> MLTEGISIQSYDGHTFGALVGSPAKAPAPVIVIAHEILGVNAFM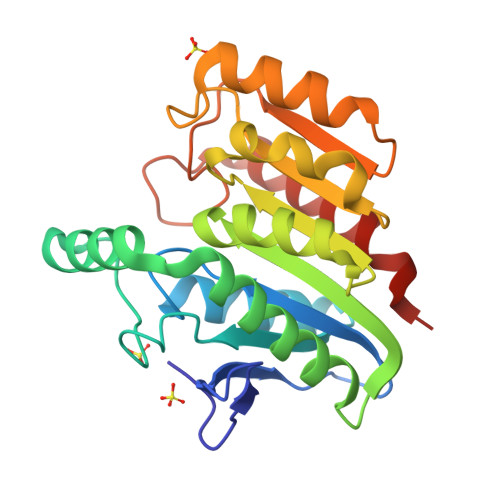RETVSWLVDQGYAAVCPDLHARQAPGTALDPLDEAQREQAYKLWQAFDMEAGVGDLEAAIRYARHLPYSNGKVGLVGYSLGGALAFLVAAKGCVDRVVGYCGVGLEKQLDKVPEVKHPALFHMGGQDHFVPAPSRQLITEGFGANPLLQVHWYEGAGHSFARTGSSDYVASAAALANERTLDFLAPLQGKKPQ>SNAMHFSIPETESRSGDSGGSAYVAYNIHVNGVLHCRVRYSQLLGLHEQLRKEYGANVLPAFPPKKLFSLTPAEVEQRREQLEKYMQAVR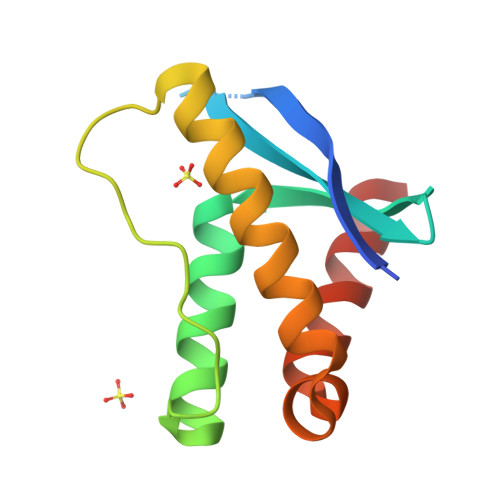QDPLLGSSETFNSFLRRAQQETQQV[3x]> GAMGGAHKVRAGGPGLERAEAGVPAEFSIWTREAGAGGLAIAVEGPSKAEISFEDRKDGSCGVAY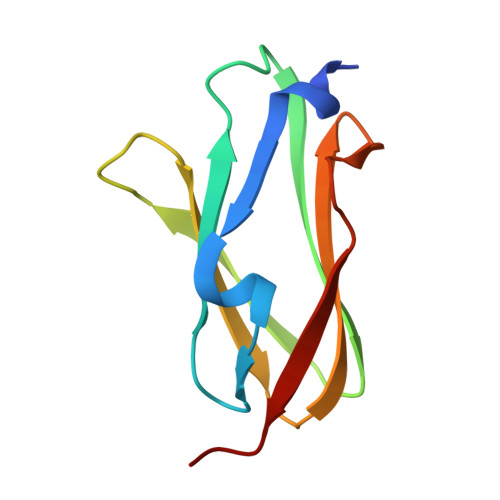VVQEPGDYEVSVKFNEEHIPDSPFVVPVASPS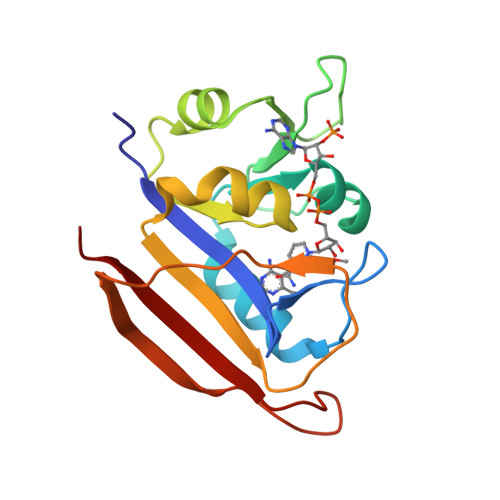>[2x]HHHMRVSFMVAMDENRVIGKDNNLPWRLPSELQYVKKTTMGHPLIMGRKNYEAIGRPLPGRRNIIVTRNEGYHVEGCEVAHSVEEVFELCKNEEEIFIFGGAQIYDLFLPYVDKLYITKIHHAFEGDTFFPEMDMTNWKEVFVEKGLTDEKNPYTYYYHVYEKQQ RNF213, also known as ‘mysterin’, is the major susceptibility gene for Moyamoya disease (MMD), a cerebrovascular disorder characterized by arterial occlusions and abnormal blood vessel generation. Notably, with a mass of 591 kDa, RNF213 is the largest E3 ubiquitin ligase in the human proteome. It combines RING and AAA (ATPase associated with a variety of cellular activities) domains in a single polypeptide, making it a unique E3 machine in the ubiquitination system. As seen in the high-resolution cryo-EM structure, the 584 kDa RNF213 protein adopts an intricately intertwined fold that is organized into three major modules, namely an N-terminal stalk, a dynein-like core with six AAA units, and a multidomain E3 module.

The final atomic models of wildtype (wt) RNF213 and the R4753K MMD mutant comprise residues 476–5148, contain >80% of all side chains and were resolved at an average resolution of 3.2 Å and 3.1 Å, respectively, with the best-refined regions reaching 2.8 Å. We concentrated our analysis on the human R4810K founder mutation, the most widespread disease variant present in more than 2.0% of the East Asian population. Cryo-EM analysis of the equivalent R4753K mutation in mouse RNF213 indicated that wt and R4753K proteins have an almost identical structure and can be aligned with a root mean square (rms) deviation of 0.69 Å for 4308 Cα atoms. Arg4753 is located at the end of an α-helix, fastening the ends of an ‘omega’ structure formed by residues 4750–4809. Asp4806, the partner residue on the opposite flank of this motif, undergoes close interactions with Arg4753, as directly seen in the cryo-EM density. The R4753K mutation disrupts this salt bridge, weakening the sealing of the omega motif and leading to small but significant structural adaptations in its immediate environment. Interestingly, mutating the Arg4753 partner residue Asp4806 is also associated with MMD, highlighting the relevance of the identified structural motif. To functionally characterize R4753K, we performed ATPase and ubiquitination assays. These data indicated that the MMD founder mutation, though causing local structural changes, does not significantly alter the enzymatic properties of RNF213 in vitro. Consistent with the minor structural and functional effects, the penetrance of R4753K in MMD is low, as only 1 from 200 carriers develops disease.

> XXXXXXXXXXXXXXXXXXXXXXXXXXXXXXXXXXXXXXXXXXXXXXXXXXXXXXXXXXXXXXXXXXXKLTLGLSILFMVEAAEFTVPKKDLDSLCYLLIPSAGSPEALHSDLSPVLRIRQRWRIYLTNLCLRCIDERCDRWLGILPLLHTCMQKSPPKKNSKSQPEDTWAGLEGISFSEFRDKAPTRSQPLQFMQSKMALLRVDEYLFRSWLSVVPLESLSSYLENSIDYLSDVPVRVLDCLQGISYRLPGLRKISNQNMKKDVENVFKMLMHLVDIYQHRIFGENLLQIYLTECLTLHETVCNITANHQFFEIPALSAELICKLLELSPPGHTDEGLPEKSYEDLVTSTLQEALATTRNWLRSLFKSRMLSISSAYVRLTYSEEMAVWRRLVEIGFPEKHGWKGSLLGDMEGRLKQEPPRLQISFFCSSQCRDGGLHDSVSRSFEKCVIEAVSSACQSQTSVLEGLSCQDLQKFGTLLSAVITKSWPVHNGEPVFDVDEIFKYLLKWPDVRQLFELCGTNEKIIDNITEEGRQLMATAESVFQKVAGELENGTIVVGQLELILEHQSQFLDIWNLNRRRLPSQEKACDVRSLLKRRRDDLLFLKQEKRYVESLLRQLGRVKHLVQVDFGNIEIIHSQDLSNKKLNEAVIKLPNSSSYKRETHYCLSPDIREMASKLDSLKDSHIFQDFWQETAESLNTLDKDPRELKVSLPEVLEYLYNPCYDNFYTLYENLKSGKITFAEVDAIFKDFVDKYDELKNDLKFMCTMNPQDQKGWISERVGQIKEYHTLHQAVSSAKVILQVRRALGVTGDFSVLNPLLNFADSFEDFGNEKLDQISPQFIKAKQLLQDISEPRQRCLEELARQTELVAWLHKALEDINELKVFVDLASISAGENDIDVDRVACFHDAVQGYASLLYKMDERTNFSDFMNHLQELWRALDNDQHLPDKLKDSARNLEWLKTVKESHGSVELSSLSLATAINSRGVYVIEAPKDGQKISPDTVLRLLLPDGHGYPEALRTYSTEELKELLNKLMLMSGKKDHNSNTEVEKFSEVFSNMQRLVHVFIKLHCAGNMLFRTWTAKVYCCPDGGIFMNFGLELLSQLTEKGDVIQLLGALCRQMEDFLDNWKTVVAQKRAEHFYLNFYTAEQLVYLSSELRKPRPSEAALMMLSFIKGKCTVQDLVQATSACESKADRYCLREVMKKLPQQLLSEPSLMGKLQVIMMQSLVYMSAFLPHCLDLDALGRCLAHLATMGGTPVERPLPKGLQAGQPNLILCGHSEVLPAALAIYMQAPRQPLPTFDEVLLCTPATTIEEVELLLRRCLTSGSQGHKVYSLLFADQLSYEVGCQAEEFFQSLCTRAHREDYQLVILCDAAREHCYIPSTFSQYKVPLVPQAPLPNIQAYLQSHYQVPKRLLSAATVFRDGLCVGIVTSERAGVGKSLYVNTLHTKLKAKLRDETVPLKIIRLTEPHLDENQVLSALLPFLKEKYQKMPVIFHIDISTSVQTGIPIFLFKLLILQYLMDINGKIWRRSPGHLYLVEIPQGLSVQPKRSSKLNARAPLFKFLDLFPKVTCRPPKEVIDMELTPERSHTDPAMDPVEFCSEAFQRPYQYLKRFHQQQNLDTFQYEKGSVEGSPEECLQHFLIYCGLINPSWSELRNFAWFLNCQLKDCEASIFCKSAFTGDTLRGFKNFVVTFMILMARDFATPTLHTSDQSPGRQSVTIGEVVEEDLAPFSLRKRWESEPHPYVFFNGDHMTMTFIGFHLETNNNGYVDAINPSNGKVIKKDVMTKELFDGLRLQRVPFNIDFDNLPRYEKLERLCLALGIEWPIDPDETYELTTDNMLKILAIEMRFRCGIPVIIMGETGCGKTRLIKFLSDLKRGSVEAETMKLVKVHGGTTPSMIYSKVKEAERTAFSNKAQHKLDTILFFDEANTTEAVSCIKEILCDRTVDGEHLHEDSGLHIIAACNPYRKHSQEMILRLESAGLGYRVSAEETADRLGSIPLRQLVYRVHALPPSLIPLVWDFGQLNDSAEKLYIQQIVQRLVDSVSVNPSETCVIADVLSASQMFMRKRENECGFVSLRDVERCVKVFRWFHDHSDMLLKELDKFLHESSDSTHTFERDPVLWSLVMAIGVCYHASLEEKASYRTAIARCFPKPYNSSRAILDEVTHVQDLFLRGAPIRTNIARNLALKENVFMMVICIELKIPLFLVGKPGSSKSLAKIIVADAMQGQAAFSELFRCLKQVHLVSFQCSPHSTPQGIISTFKQCARFQQGKDLGQYVSVVVLDEVGLAEDSPKMPLKTLHPLLEDGCIEDDPAPYKKVGFVGISNWALDPAKMNRGIFVSRGSPNEKELIESAEGICSSDRLVQDKIRGYFAPFAKAYETVCQKQDKEFFGLRDYYSLIKMVFAKAKASKRGLSPQDITHAVLRNFSGKDNIQALSIFTASLPEARYKEEVSTVELIKQNIYPGPQASSRGLDGAESRYLLVLTRNYVALQILQQTFFEGQQPEIIFGSSFPQDQEYTQICRNINRVKICMETGKMVVLLNLQNLYESLYDALNQYYVYLGGQKYVDLGLGTHRVKCRVHTAFRLIVIEEKDVVYKQFPVPLINRLEKHYLDMNTVLQPWQKSIVQELQQWAHEFADVKADQFIARHKYSPADVFIGYHSDACASVVLQAVERQGCRDLTEELYRKVSEEARSILLDCATPDAVVRLSGSSLGSFTAKQLSQEYYYAQQHNSFVDFLQAHLRMTHHECRAVFTEITTFSRLLTGNDCDVLASELRGLASKPVVLSLQQYDTEYSFLKDVRSWLTNPGKRKVLVIQADFDDGTRSAQLVASAKYTAINEINKTQGTKDFVFVYFVTKLSRMGSGTSYVGFHGGLWRSVHIDDLRRSTIMASDVTKLQNVTISQLFKPEDKPEQEEMEIETSQSKELAEEQMEVEDSEEMKKASDPRSCDCSQFLDTTRLVQSCVQGAVGMLRDQNESCARNMRRVTILLDLLNEDNTRNASFLRESKMRLHVLLNKQEENQVRSLKEWVTREAANQDALQEAGTFRHTLWKRVQDVVTPILASMIAHIDRDGNLELLAQPDSPAWVQDLWMFIYSDIKFLNISLVLNNTRSNSEMSFILVQSHMNLLKDAYNAVPFSWRIRDYLEELWVQAQYITDTEGLSKKFVEIFQKTPLGVFLAQFPVAQQQKLLQSYLKDFLLLTMKVSSREELMFLQMALWSCLRELQEASGTPDETYKFPLSLPWVHLAFQHFRTRLQNFSRILTIHPQVLSSLSQAAEKHSLAGCEMTLDAFAAMACAEMLKGDLLKPSPKAWLQLVKNLSTPLELVCSEGYLCDSGSMTRSVIQEVRALWNRIFSIALFVEHVLLGTESHIPELSPLVTTYVSLLDKCLEEDSNLKTCRPFVAVMTTLCDCKDKASKKFSRFGIQPCFICHGDAQDPVCLPCDHVYCLRCIQTWLIPGQMMCPYCLTDLPDKFSPTVSQDHRKAIEKHAQFRHMCNSFFVDLVSTMCFKDNTPPEKSVIDTLLSLLFVQKELLRDASQKHREHTKSLSPFDDVVDQTPVIRSVLLKLLLKYSFHEVKDYIQNYLTQLEKKAFLTEDKTELYLLFISCLEDSVHQKTSAGCRNLEQVLREEGHFLRTYSPGLQGQEPVRIASVEYLQEVARVRLCLDLAADFLSELQEGSELAEDKRRFLKHVEEFCTRVNNDWHRVYLVRKLSSQRGMEFVQSFSKQGHPCQWVFPRKVIAQQKDHVSLMDRYLVHGNEYKAVRDATAKAVLECKTLDIGNALMACRSPKPQQTAYLLLALYTEVAALYRSPNGSLHPEAKQLEAVNKFIKESKILSDPNIRCFARSLVDNTLPLLKIRSANSILKGTVTEMAVHVATILLCGHNQILKPLRNLAFYPVNMANAFLPTMPEDLLVHARTWRGLENVTWYTCPRGHPCSVGECGRPMQESTCLDCGLPVGGLNHTPHEGFSAIRNNEDRTQTGHVLGSPQSSGVAEVSDRGQSPVVFILTRLLTHLAMLVGATHNPQALTVIIKPWVQDPQGFLQQHIQRDLEQLTKMLGRSADETIHVVHLILSSLLRVQSHGVLNFNAELSTKGCRNNWEKHFETLLLRELKHLDKNLPAINALISQDERISSNPVTKIIYGDPATFLPHLPQKSIIHCSKIWSCRRKITVEYLQHIVEQKNGKETVPVLWHFLQKEAELRLVKFLPEILALQRDLVKQFQNVSRVEYSSIKGFIHSHSSDGLRKLLHDRITIFLSTWNALRRSLETNGEIKLPKDYCCSDLDLDAEFEVILPRRQGLGLCGTALVSYLISLHNNMVYTVQKFSNEDNSYSVDISEVADLHVISYEVERDLNPLILSNCQYQVQQGGETSQEFDLEKIQRQISSRFLQGKPRLTLKGIPTLVYRRDWNYEHLFMDIKNKMAQSSLPNLAISTISGQLQSYSDACEALSIIEITLGFLSTAGGDPGMDLNVYIEEVLRMCDQTAQVLKAFSRCQLRHIIALWQFLSAHKSEQRLRLNKELFREIDVQYKEELSTQHQRLLGTFLNEAGLDAFLLELHEMIVLKLKGPRAANSFNPNWSLKDTLVSYMETKDSDILSEVESQFPEEILMSSCISVWKIAATRKWDRQSRGGGHHHHHHHHHH2-benzyl-5-nitro-1H-benzimidazole | C14 H11 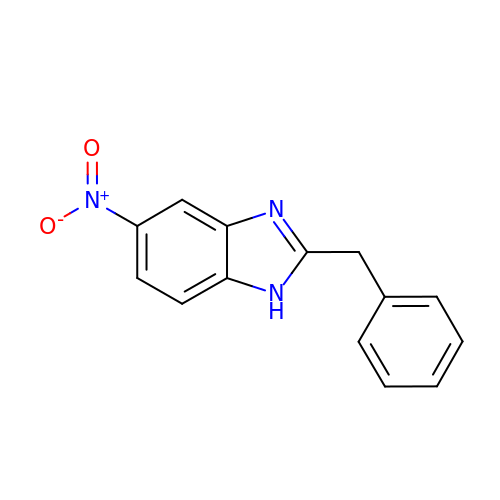N3 O2 | UMWIVOZCYNITGG-UHFFFAOYSA-N>GSPQAHPVPKDARITHSSGQSFEQMRQECLQRGTLFEDADFPASNSSLFYSERPQIPFVWKRPGEIVKNPEFILGGATRTDICQGELGDCWLLAAIASLTLNQKALARVIPQDQSFGPGYAGIFHFQFWQHSEWLDVVIDDRLPTFRDRLVFLHSADH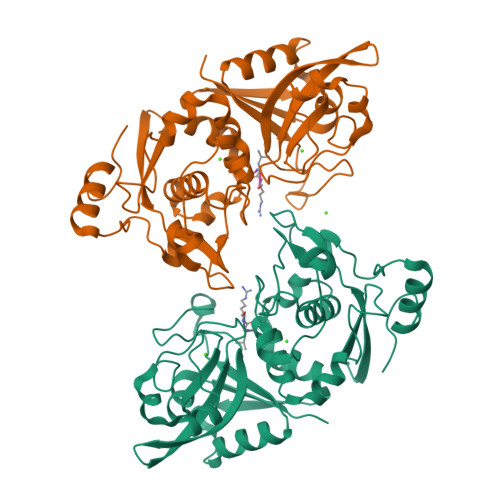NEFWSALLEKAYAKLNGSYEALKGGSAIEAMEDFTGGVAETFQTKEAPENFYEILEKALKRGSLLGCFIDTRSAAESEARTPFGLIKGHAYSVTGIDQVSFRGQRIELIRIRNPWGQVEWNGSWSDSSPEWRSVGPAEQKRLCHTALDDGEFWMAFKDFKAHFDKVEICNLTPDA[2x]>FDDLRPRLGRLTEETIDIAREVLVEGKSQSDVARERGLSRQRVSSMVKSVVSAANEIPREWQRVEVWLPPNLAEKVRQMEADAKADVARK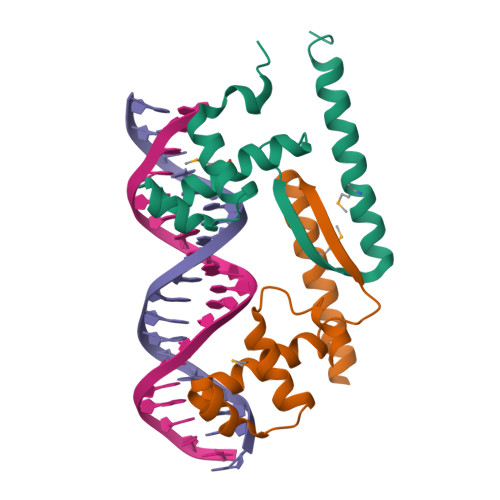NQLTDAAL[2x]> MALVDGFLELERSSGKLEWSAILQKMASDLGFSKILFGLLPKDSQDYENAFIVGNYPAAWREHYDRAGYARVDPTVSHCTQSVLPIFWEPSIYQTRKQHEFFEEASAAGLVYGLTMPLHGARGELGALSLSVEAENRAEA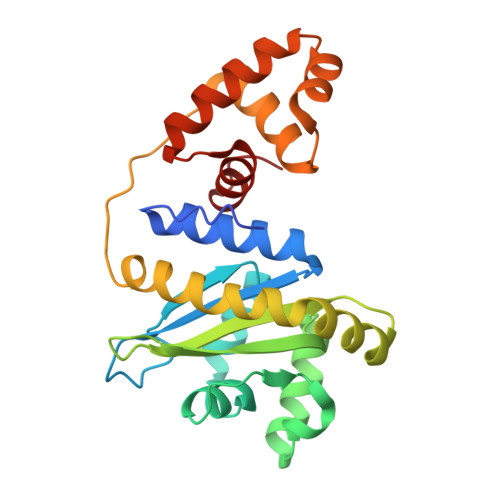NRFMESVLPTLWMLKDYALQSGAGLAFEHPVSKPVVLTSREKEVLQWCAIGKTSWEISVICNCSEANVNFHMGNIRRKFGVTSRRVAAIMAVNLGLITL>[2x]AGTPDPLITEIQPWASEFGEAVDAHPYGLPIHFESHVKRQYVEWLTESPVSSINFTPIHALEGTITPQGCAFERHHSGAIELSKQDYRLMINGLVEKPLVFTFEDLLRFPRTTTTAFCECAANGGMEWGGAQLEGCQYTQGMIHNMEYVGVPLSVLLAEAGVKPEGKWLYAEGADASSNGRSFPMEKVMDDVMLAFFANGEALRKEHGYPARLVVPGWEGNMWVKWVRRLGIYDKAVESREETSKYTD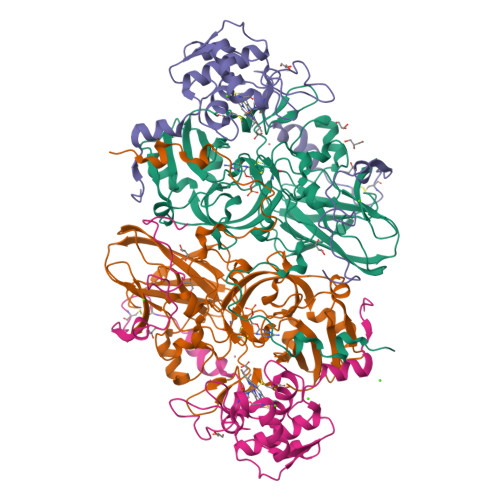LMPDGRARKWTWVMDAKSVITSPSPQVPIRHGKGPLVISGLAWSGNGRITRVDVSLDGGKNWTTARITGQALPKALTRFHLDIDWDGSEMLLQSRAVDETGYVQPTKDALRAIRGRNNVYHNNGIQTWWVKADGEVENVEIA;>[2x]DKLGLGREALPEEISAWDTAVLPDGQGLRPGSGDVATGDALFADNCASCHGDFAEGLDSWPVLAGGDGSLTDPRPVKTIGSYWPYLSTVYDYVHRSMPFGSAQTLSVDDTYAITAFLLYSNGLVEDDFVLTHENFTQVVLPNAEGFYPDDRDQTEYPLFSKEPCMTDCAVGVEITKRAVDLNVTPEDPDGRPAGSMPDLGAAAAP> MTTTMKISIEFLEPFRMTKWQESTRRNKNNKEFVRGQAFARWHRNKKDNTKGRPYITGTLLRSAVIRSAENLLTLSDGKISEKTCCPGKFDTEDKDRLLQLRQRSTLRWTDKNPCPDNAETYCPFCELLGRSGNDGKKAEKKDWRFRIHFGNLSLPGKPDFDGPKAIGSQRVLNRVDFKSGKAHDFFKAYEVDHTRFPRFEGEITIDNKVSAEARKLLCDSLKFTDRLCGALCVIRFDEYTPAADSGKQTENVQAEPNANLAEKTAEQIISILDDNKKTEYTRLLADAIRSLRRSSKLVAGLPKDHDGKDDHYLWDIGKKKKDENSVTIRQILTTSADTKELKNAGKWREFCEKLGEALYLKSKDMSGGLKITRRILGDAEFHGKPDRLEKSRSVSIGSVLKETVVCGELVAKTPFFFGAIDEDAKQTDLQVLLTPDNKYRLPRSAVRGILRRDLQTYFDSPCNAELGGRPCMCKTCRIMRGITVMDARSEYNAPPEIRHRTRINPFTGTVAEGALFNMEVAPEGIVFPFQLRYRGSEDGLPDALKTVLKWWAEGQAFMSGAASTGKGRFRMENAKYETLDLSDENQRNDYLKNWGWRDEKGLEELKKRLNSGLPEPGNYRDPKWHEINVSIEMASPFINGDPIRAAVDKRGTDVVTFVKYKAEGEEAKPVCAYKAESFRGVIRSAVARIHMEDGVPLTELTHSDCECLLCQIFGSEYEAGKIRFEDLVFESDPEPVTFDHVAIDRFTGGAADKKKFDDSPLPGSPARPLMLKGSFWIRRDVLEDEEYCKALGKALADVNNGLYPLGGKSAIGYGQVKSLGIKGDDKRISRLMNPAFDETDVAVPEKPKTDAEVRIEAEKVYYPHYFVEPHK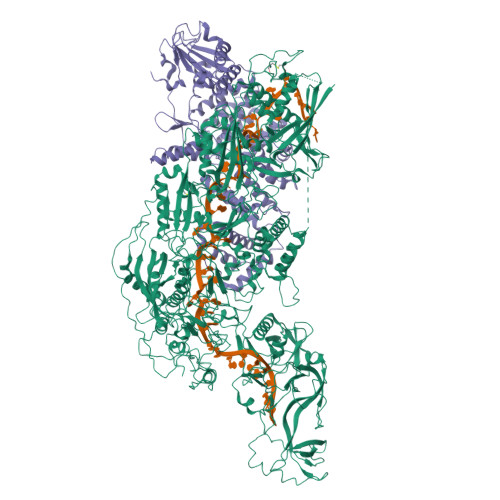KVEREEKPCGHQKFHEGRLTGKIRCKLITKTPLIVPDTSNDDFFRPADKEARKEKDEYHKSYAFFRLHKQIMIPGSELRGMVSSVYETVTNSCFRIFDETKRLSWRMDADHQNVLQDFLPGRVTADGKHIQKFSETARVPFYDKTQKHFDILDEQEIAGEKPVRMWVKRFIKRLSLVDPAKHPQKKQDNKWKRRKEGIATFIEQKNGSYYFNVVTNNGCTSFHLWHKPDNFDQEKLEGIQNGEKLDCWVRDSRYQKAFQEIPENDPDGWECKEGYLHVVGPSKVEFSDKKGDVINNFQGTLPSVPNDWKTIRTNDFKNRKRKNEPVFCCEDDKGNYYTMAKYCETFFFDLKENEEYEIPEKARIKYKELLRVYNNNPQAVPESVFQSRVARENVEKLKSGDLVYFKHNEKYVEDIVPVRISRTVDDRMIGKRMSADLRPCHGDWVEDGDLSALNAYPEKRLLLRHPKGLCPACRLFGTGSYKGRVRFGFASLENDPEWLIPGKNPGDPFHGGPVMLSLLERPRPTWSIPGSDNKFKVPGRKFYVHHHAWKTIKDGNHPTTGKAIEQSPNNRTVEALAGGNSFSFEIAFENLKEWELGLLIHSLQLEKGLAHKLGMAKSMGFGSVEIDVESVRLRKDWKQWRNGNSEIPNWLGKGFAKLKEWFRDELDFIENLKKLLWFPEGDQAPRVCYPMLRKKDDPNGNSGYEELKDGEFKKEDRQKKLTTPWTPWA;> MSNPIRDIQDRLKTAKFDNKDDMMNLASSLYKYEKQLMDSSEATLCQQGLSNRPNSFSQLSQFRDSDIQSKAGGQTGKFWQNEYEACKNFQTHKERRETLEQIIRFLQNGAEEKDADDLLLKTLARAYFHRGLLYRPKGFSVPARKVEAMKKAIAYCEIILDKNEEESEALRIWLYAAMELRRCGEEYPENFAEKLFYLANDGFISELYDIRLFLEYTEREEDNNFLDMILQENQDRERLFELCLYKARACFHLNQLNDVRIYGESAIDNAPGAFADPFWDELVEFIRMLRNKKSELWKEIAIKAWDKCREKEMKVGNNIYLSWYWARQRELYDLAFMAQDGIEKKTRIADSLKSRTTLRIQELNELRKDAHRKQNRRLEDKLDRIIEQENEARDGAYLRRNPPCFTGGKREEIPFARLPQNWIAVHFYLNELESHEGGKGGHALIYDPQKAEKDQWQDKSFDYKELHRKFLEWQENYILNEEGSADFLVTLCREIEKAMPFLFKSEVIPEDRPVLWIPHGFLHRLPLHAAMKSGNNSNIEIFWERHASRYLPAWHLFDPAPYSREESSTLLKNFEEYDFQNLENGEIEVYAPSSPKKVKEAIRENPAILLLLCHGEADMTNPFRSCLKLKNKDMTIFDLLTVEDVRLSGSRILLGACESDMVPPLEFSVDEHLSVSGAFLSHKAGEIVAGLWTVDSEKVDECYSYLVEEKDFLRNLQEWQMAETENFRSENDSSLFYKIAPFRIIGFPAE> MAPVKVFGPAMSTNVARVTLCLEEVGAEYEVVNIDFNTMEHKSPEHLARNPFGQIPAFQDGDLLLWESRAISKYVLRKYKTDEVDLLRESNLEEAAMVDVWTEVDAHTYNPALSPIVYQCLFNPMMRGLPTDEKVVAESLEKLKKVLEVYEARLSKHSYLAGDFVSFADLNHFPYTFYFMATPHAALFDSYPHVKAWWDRLMARPAVKKIAATMVPPKACLFAESLEKLKKVLEVYEARLSKHSYLAGDFVSFADLNHFPYTFYFMATPHAALFDSYPHVKAWWDRLMARPAVKKIAATMVPPKA

In black-grass, upregulation of a phi (F)-class GST1 (AmGSTF1) has been shown to be a functional biomarker of MHR. Recombinant AmGSTF1 has been shown to exhibit both glutathione-S-transferase activity toward xenobiotics, as well as acting as a GPOX, reducing fatty-acid hydroperoxides to less reactive monohydroxy derivatives. The Phi (F) class GSTs, of which AmGSTF1 is an example, are found in all higher plants, being homodimeric enzymes in which each protomer of approximately 23–30 kDa with the catalytic serine residues located at the interface. Each protomer has two distinct domains; the N-terminal domain adopts the typical thioredoxin-fold, with the C-terminal domain being a bundle of at least five helices as demonstrated by the crystal structures of AmGSTF1 presented here.

Importantly, just as treatment of MHR black-grass plants with NBD-Cl reversed resistance toward three herbicide chemistries, this alkylating agent also disrupts the drug resistance function of HsGSTP1 in human tumour cells. In both cases, the inhibitory activity of NBD-Cl was linked to the alkylation of specific cysteine residues, namely Cys47 in HsGSTP1 and Cys120 in AmGSTF1, which are respectively located on opposite sides of the binding cleft in different loop regions of each protein (Fig. S1b‡). To determine the structural basis of this covalent modification, AmGSTF1 was quantitatively alkylated with NBD-Cl as confirmed by mass spectrometric analysis prior to crystallisation (data not shown). The modified protein crystallised in the same hexagonal space group as the native form, diffracting to 2.8 Å, revealing a conformation that is almost identical in structure to the apo-protein, with rmsd of 0.2 Å for 188 Cα-atoms. The Cys120-NBD adduct was clearly visible in the unbiased electron density (Fig. S3‡), even though the density and the refinement indicated only partial occupancy in the crystal. Although not directly associated with the active site, Cys120 is one of the last residues visible prior to the disordered loop projecting into the active site of the neighbouring polypeptide subunit. The alkylated residue points into the H-site of the symmetry-related protein. The covalent modification of cysteines located in the binding loop clearly affect enzymatic activity presumably due to changes in dynamic behaviour.> PKVSVLITVTGVDQPGVTATLFEVLSRHGVELLNVEQVVIRHRLTLGVLVCCPADVADGPALRHDVEAAIRKVGLDVSIERSDDVPIIREPSTHTIFVLGRPITAAAFGAVAREVAALGVNIDLIRGVSDYPVIGLELRVSVPPGADGALRTALNRVSSEEHVDVAVEDYTLERRAKRLIVFDVDSTLVQGEVIEMLAAKAGAEGQVAAITDAAMRGELDFAQSLQQRVATLAGLPATVIDEVAGQLELMPGARTTLRTLRRLGYACGVVSGGFRRIIEPLAEELMLDYVAANELEIVDGTLTGRVVGPIIDRAGKATALREFAQRAGVPMAQTVAVGDGANDIDMLAAAGLGIAFNAKPALRE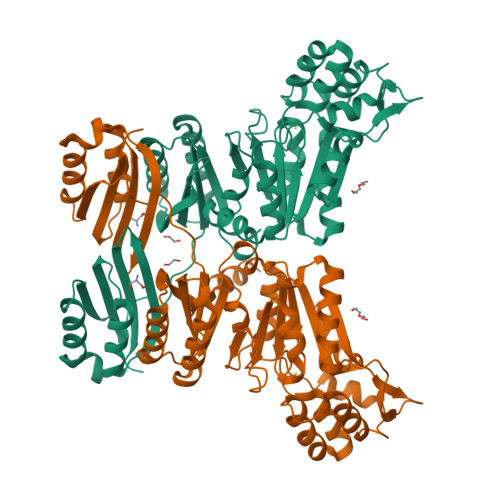VADASLSHPYLDTVLFLLGVTRGEIEAADAID> MTDAVLELPAATFDLPLSLSGGTQTTLRAHAGHWLVIYFYPKDSTPGCTTEGLDFNALLPEFDKAGAKILGVSRDSVKSHDNFCAKQGFAFPLVSDGDEALCRAFDVIKEKNMYGKQVLGIERSTFLLSPEGQV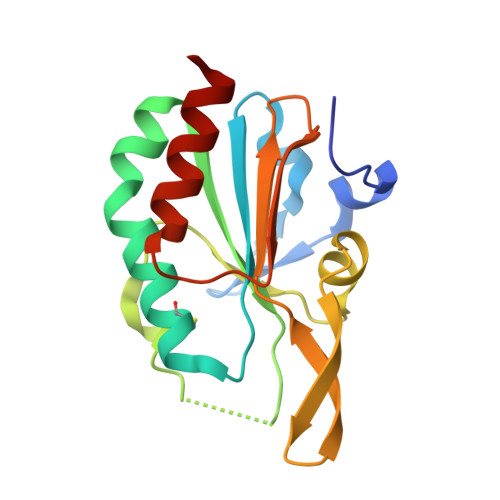VQAWRKVKVAGHADAVLAALKAHAKQ>[6x]MAHHHHHHMEKSFIMIKPDGVQRGLVGTIIKRFEKKGYKLIAIKMLNPTEEILKEHYKELSDQP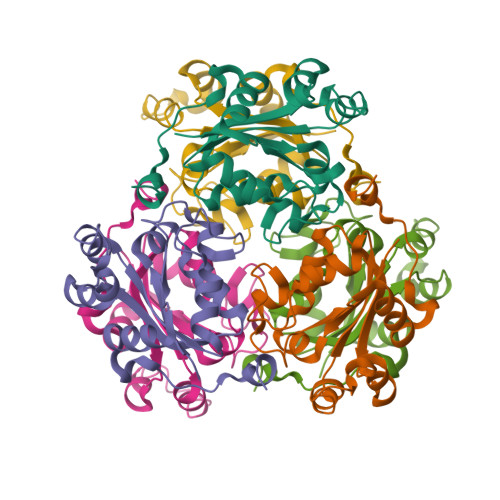FFKNLVAYISKGPVVAMVWEGVDMVKQGRKLIGETNPLTSNTGTIRGDFCLEVSKNVIHGSDSVASANKEINIWFKAEELTQWKHHMKEWICS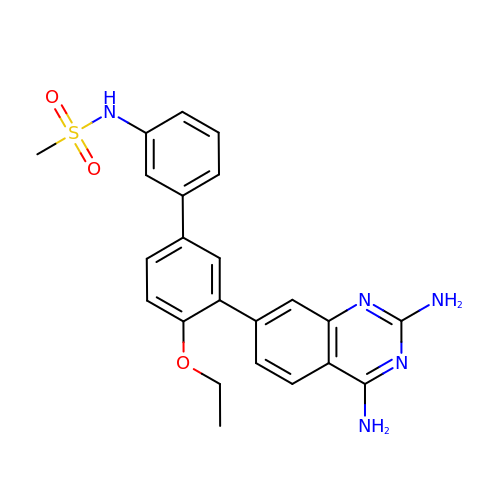N-[3'-(2,4-diaminoquinazolin-7-yl)-4'-ethoxybiphenyl-3-yl]methanesulfonamide | C23 H23 N5 O3 S | KBZJKRXRDPRBNM-UHFFFAOYSA-N>MAHHHHHHSSGLEVLFQGPMTHSVVELIEI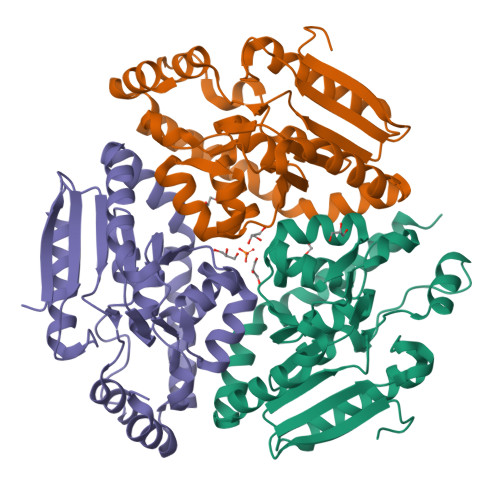ESAIIQVKMQDRTHKNAFSQELTDDLIQAFEYIRQNPKYKAVILTGYDNYFASGGTQEGLLRIQQGLTKFTDDNLYSLALDCEIPVIAAMQGHGIGGGFVMGLFADIVILSRESVYTANFMKYGFTPGMGATFIVPKKLGFSLAQEILLNAGSYRGADLEKRGVPFKVLPRAEVLDYAVELAQELAEKPRNSLVTLKDHLVAPLRDQLPRVIEQELMMHEATFHHEEVKSRIKGLYGN[3x]> GSNGMSQLPAPVSVESSWRYIDTQGQIHGPFTTQMMSQWYIGGYFASTLQISRLGSTPETLGINDIFITLGELMTKLEKYDTDPFTTFDKLHVQTTSS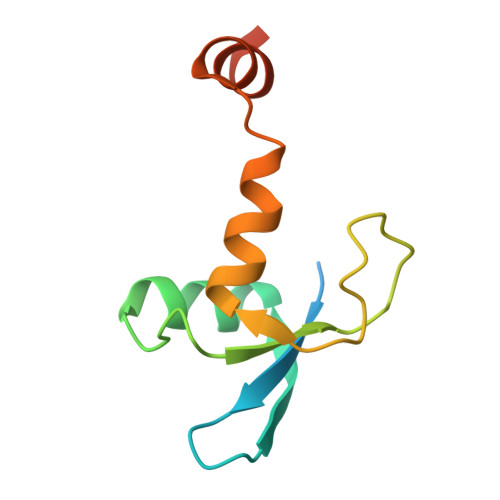DS> MANPRVMDKCKKVYENYPVSKCQLANQCNYDCKLDKHARSG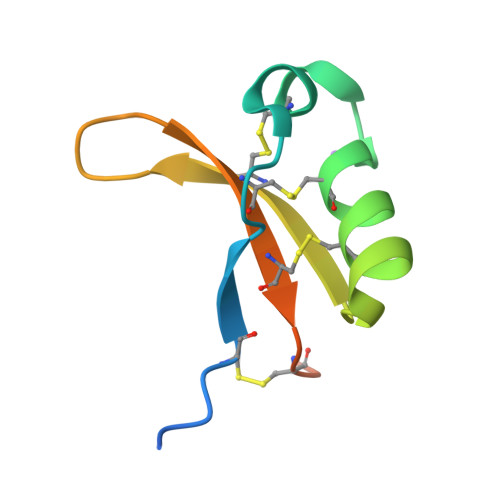ECFYDEKANLQCICDYCEYPLEHHHHHH>SMVEYTKESVQADPENWRSVDPDNLVIFETTKGVVYIEL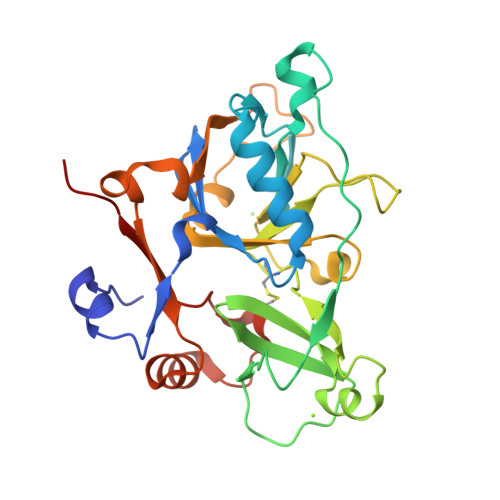APEIAPNHVAQIRKVVRTGLYSGTKFHRVISGFMAQGGDIAATLGREPDLEAVDGEFVFRRDPKSIVLTVINEEDQTKSQYTGFYNGFPIETRQDELANYSEDKRVESWMPHCAGVVSMARTNDPNSGKDQFFLMRDESRFLDRKYSSWGRMLEGLDVAKSLTIGEPPERPDILVSAVMVSDLAPKDRPEAWVMRNDGPMFSLFLDRMGRDKDVCSLPQTPSVVFVSEDKEG[2x]> FPTIPLSRLFDNAMLRAHRLHQLAFDTYQEFEEAYIPKEQKYSFLQNPQ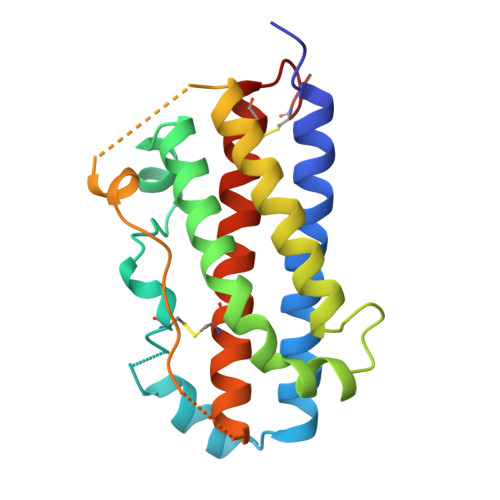TSLCFSESIPTPSNREETQQKSNLELLRISLLLIQSWLEPVQFLRSVFANSLVYGASDSNVYDLLKDLEERIQTLMGRLTDGSPRTGQIFKQTYSKFDTNSHNDDALLKNYGLLYCFRRDMTYVATYLRIVQCRSVEGSCGF>GKEQPQVRGELEETQETQEDGNSTQRTTPVSVNYHFTRQCNYKCGFCFHTAKTSFVLPLEEAKRGLLLLKQAGLEKINFSGGEPFLQDRGEYLGKLVRFCKEELALPSVSIVSNGSLIRERWFKDYGEYLDILAISCDSFDEQVNALIGRGQGKKNHVENLQKLRRWCRDYKVAFKINSVINRFNVDEDMNEHIKALSPVRWKVFQCLLIEGENSGADALRAAERFLISNEEFETFLERHKEVSCLVPESNQKMKDSYLILDEYMRFLNCTGGRKDPSKSILDVGVEEAIKFSGFDEKMFL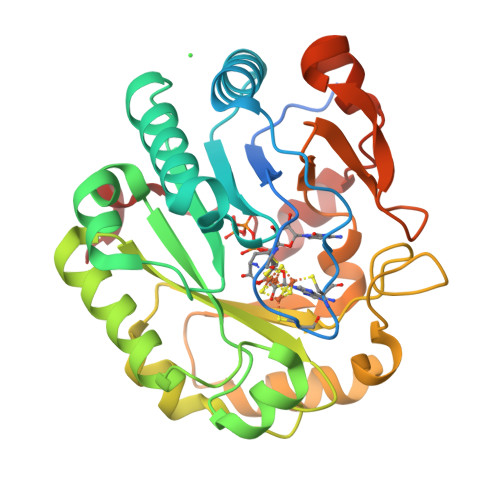KRGGKYVWSKADLKLDW[2x]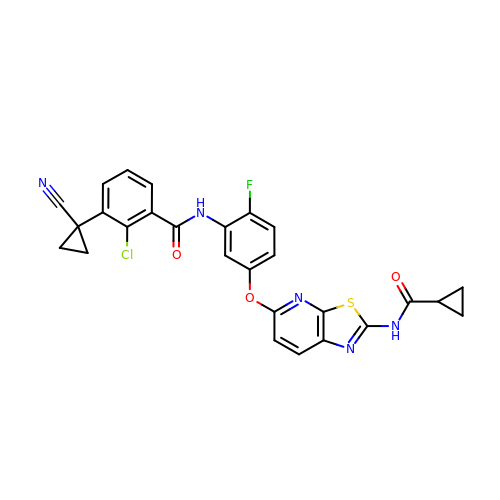2-chloro-3-(1-cyanocyclopropyl)-N-[5-({2-[(cyclopropylcarbonyl)amino][1,3]thiazolo[5,4-b]pyridin-5-yl}oxy)-2-fluorophenyl]benzamide | C27 H19 Cl F N5 O3 S | MDPMAXSABUPRJI-UHFFFAOYSA-N>[2x]MPKRLGFFTRLLDQGSAQTRYRLAAEQIRHAERVGFDSAWIAQHHFHEQEGGLPSPLVFLAHVAAQTDRIRLGTAIITLPMENPLRVAEDAAVLDLLT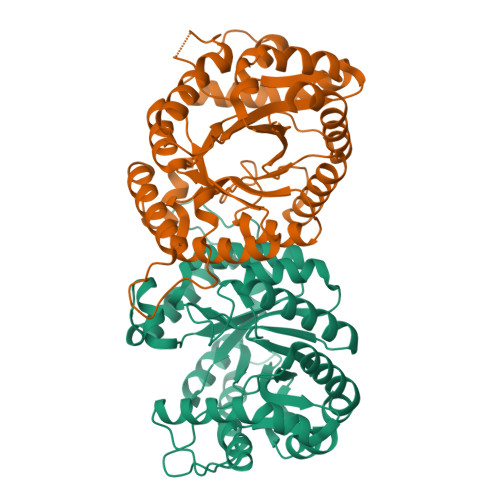DGRLEVGFGSGGTPTSFLPFGLTSEQRGAVFADHLHLIHSAWRGDTLSHPDNHLYPPAPQLAARIWIATFSVEGAIRAGQAGHGLMLSRTQPRPPGEPRLPLDAIQNPIIDAYLSALPDGVAPRILASRTAFVADSHAHALQVAEPGLRKQAAQHREAGHRIEGDSVTDYLQQLDAHVGDPEHVIASLAQDSVLARATDISFQVHSVEPSHRDTLRSIELIAQHIAPHIR>GSHMRQDSEVNPLQVQNSSKVLNPNVTLPANNLLYDEFFVSKESKLIEDSRNNKRKTSKIASLNPYASTKAVLTTTSSTLTSDQIVVTVPQKTFIGGVYNSTTLDNLDYTPISYPLDPITVSYSFPSDFIVDTIERPSLSSMRASVFKAMRAANFSGEQSLAFDYNIKQFSYYSELKIAFGSNVNIGKIFSIDISGSNNKIKRTTGVFAKFTQKNFTIDMDLPADGNIFKNNSDLALTNGKNPVYISSVTYGRLGIISIESNASYNEVNFALKAALTAGIVNGSLNIDSNSKKILEESDLSVYLVGGRGTDAVQVIKGFAGFSNFIVNGGQFTPEAPGVPIYFSASHASDNSVYYTTFTIDK[2x]

We previously reported that Elizabethkingia anophelis, a bacterial species of the phylum Bacteroidota and a commensal of the malarial mosquito midgut produces a 2-component CDC-like (CDCL) set of proteins, encoded by adjacent genes: one large (CDCLL) and one smaller component (CDCLS). The studies herein show that, unlike their CDC relatives, the CDCLs require proteolytic activation of two distinct components that then interact and form a pore to kill bacteria using a mechanism only described for the mammalian complement membrane attack complex (MAC). The receptor for EaCDCLL or BfCDCLL is currently unknown; however, the CDCLL is the essential membrane-binding component, which recruits many CDCLS to form the β-barrel pore. This type of mechanism is only used by the complement MAC wherein a single C5b8 membrane complex recruits many C9 components to form its β-barrel pore.

The CDCLL subunit lacks the characteristic signature features for binding cholesterol, and the primary structure of the CDCLS subunit completely lacks an identifiable receptor-binding domain. The in vitro activation site for each CDCL pair resides in their regions that are analogous to the β-tongue region of the CDCs. For the EaCDCLs, proteinase K also cleaved EaCDCLL after TK66, whereas it cleaved EaCDCLS just upstream of its TK87 site after IA78. Trypsin treatment resulted in high and reproducible pore-forming activity for both the EaCDCL and BfCDCL pairs, which increased as the ratio of CDCLS to its cognate CDCLL increased and flattened at a ratio of 25–30 CDCLS to 1 CDCLL. The propeptide of the CDCLS blocks β1, which must be exposed to interact with β4 of CDCLL and of other CDCLS that oligomerize to form the β-barrel pore. The EaCDCLS alone and combined with EaCDCLL appeared as a high mass smear, which may be due to a propensity of its oligomeric complexes to form SDS-resistant aggregates.> MAQTAHQNRYQGGLCYAQCNELFSFWNPSIQQCWKGC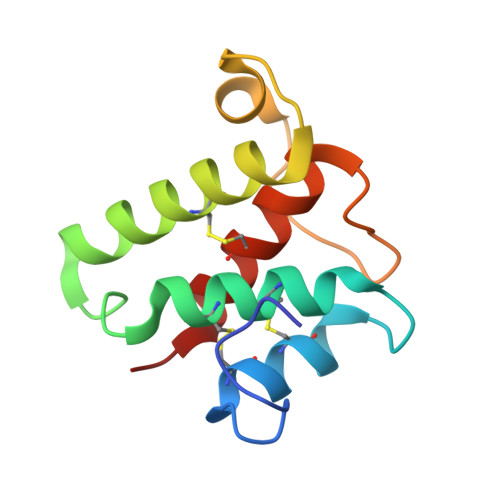DFGVGRVNDPEGRIEAQQMCKRWAAELYWTYKGELDTIKDLRVHADMYPTTPQNVYRACLAGVRRQKF~{N}-[(1~{R},2~{R},3~{R},4~{S},5~{S},6~{S})-2-(hydroxymethyl)-3,4,5,6-tetrakis(oxidanyl)cyclohexyl]pentanamide 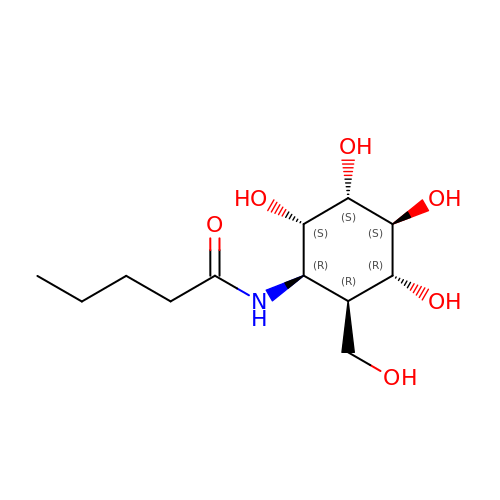| C12 H23 N O6 | MGAGNOFUGFVZSZ-MIKCJTPRSA-N> 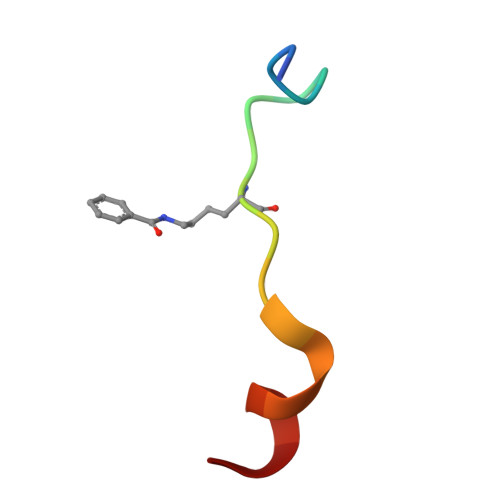TARKSTGGKAPRKQLASY3-[4-(dimethylamino)butanoylamino]-~{N}-[3-methyl-4-[(4-pyridin-3-ylpyrimidin-2-yl)amino]phenyl]benzamide 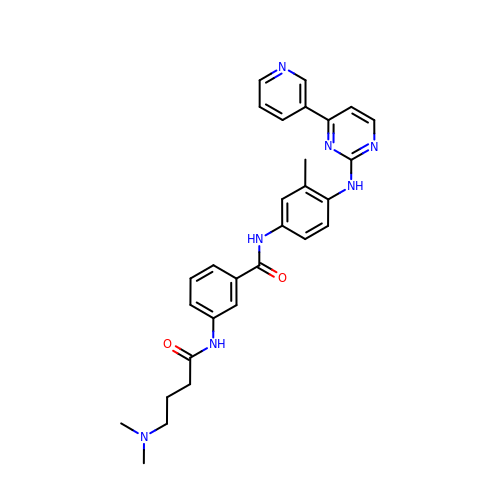| C29 H31 N7 O2 | JCQSXSKNIVAALC-UHFFFAOYSA-N>MGKTQKKNSKGRLDRYYYLAKEKGYRARSSFKIIQINEKYGHFLEKSKVVIDLCAAPGSWCQVASKLCPVNSLIIGVDIVPMKPMPNVITFQSDITTEDCRSKLRGYMKTWKADTVLHDGAPNVGLGWVQDAFTQSQLTLQALKLAVENL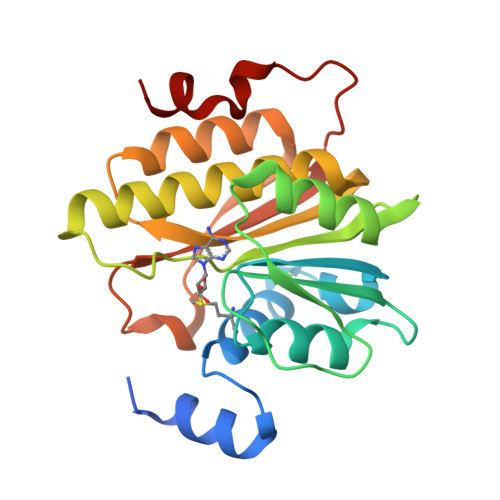VVNGTFVTKIFRSKDYNKLIWVFQQLFEKVEATKPPASRNVSAEIFVVCKGFKAPKRLDPRLLDPKEVFE[2x]>ESRTKPFTVPILTVEEMTNSRFPIPLEKLFTGPSSAFVVQPQNGRCTTDGALLGTTQLSPVDICTFRGDVTHIAGTQNYTMNLASQNWNNYDPTEEIPAPLGTPDFVGKIQGVLTQTTRRDGSTRGHKATVSTGSVHFTPKLGSVQFSTDTSNDFETGQNTRFTPVGVVQDGSTTHQNEPQQWVLPDYSGRDSHNVHLAPAVAPTFPGEQLLFFRSTMPGCSGYPNMNLDCLLPQEWVQHFYQESAPAQSDVALLRFVNPDTGRVLFECKLHKSGYVTVAHTGQHDLV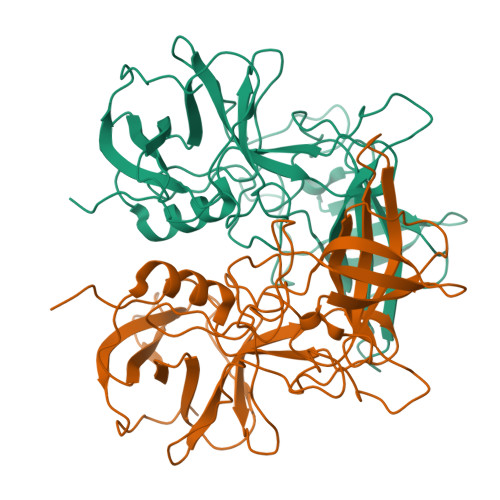IPPNGYFRFDSWVNQFYTLAPMG[10x]>EVKQENRLLNESESSSQGLLGYYFSDLNFQAPMVVTSSTTGDLSIPSSELENIPSENQYFQSAIWSGFIKVKKSDEYTFATSADNHVTMWVDDQEVINKASNSNKIRLEKGRLYQIKIQYQRENPTEKGLDFKLYWTDSQNKKEVISSDNLQLPELKQKSSNSRKKRSTSAGPTVPDRDNDGIPDSLEVEGYTVDVKNKRTFLSPWISNIHEKKGLTKYKSSPEKWSTASDPYSDFEKVTGRIDKNVSPEARHPLVAAYPIVHVDMENIILSKNEDQSTQNTDSQTRTISKNTSTSRTHTSEVHGNAEVHASFFDIGGSVSAGFSNSNSSTVAIDHSLSLAGERTWAETMGLNTADTARLNANIRYVNTGTAPIYNVLPTTSLVLGKNQTLATIKAKENQLSQILAPNNYYPSKNLAPIALNAQDDFSSTPITMNYNQFLELEKTKQLRLDTDQVYGNIATYNFENGRVRVDTGSNWSEVLPQIQETTARIIFNGKDLNLVERRIAAVNPSDPLETTKPDMTLKEALKIAFGFNEPNGNLQYQGKDITEFDFNFDQQTSQNIKNQLAELNATNIYTVLDKIKLNAKMNILIRDKRFHYDRNNIAVGADESVVKEAHREVINSSTEGLLLNIDKDIRKILSGYIVEIEDTEGLKEVINDRYDMLNISSLRQDGKTFIDFKKYNDKLPLYISNPNYKVNVYAVTKENTIINPSENGDTSTNGIKKILIFSKKGYEIG[7x];> MNEHYTESDIKRNHKTEKNKTEKEKFKDSINNLVKTEFTNETLDKIQQTQDLLKKIPKDVLEIYSELGGEIYFTDIDLVEHKELQDLSEEEKNSMNSRGEKVPFASRFVFEKKRETPKLIINIKDYAINSEQSKEVYYEIGKGISLDIISKDKSLDPEFLNLIKSLSDDSDSSDLLFSQKFKEKLELNNKSIDINFIKENLTEFQHAFSLAFSYYFAPDHRTVLELYAPDMFEYMNKLEKGGFEKISESLKKEGVEKDRIDVLKGEKALKASGLVPEHADAFKKIARELNTYILFRPVNKLATNLIKSGVATKGLNVHGKSSDWGPVAGYIPFDQDLSKKHGQQLAVEKGNLENKKSITEHEGEIGKIPLKLDHLRIEELKENGIILKGKKEIDNGKKYYLLESNNQVYEFRISDENNEVQYKTKEGKITVLGEKFNWRNIEVMAKNVEGVLKPLTADYDLFALAPSLTEIKKQIPQKEWDKVVNTPNSLEKQKGVTNLLIKYGIERKPDSTKGTLSNWQKQMLDRLNEAVKYTGYTGGDVVNHGTEQDNEEFPEKDNEIFIINPEGEFILTKNWEMTGRFIEKNITGKDYLYYFNRSYNKIAPGNKAYIEWTDPITKAKINTIPTSAEFIKNLSSIRRSSNVGVYKDSGDKDEFAKKESVKKIAGYLSDYYNSANHIFSQEKKRKISIFRGIQAYNEIENVLKSKQIAPEYKNYFQYLKERITNQVQLLLTHQKSNIEFKLLYKQLNFTENETDNFEVFQKIIDEK

Following assembly, the anthrax protective antigen (PA) forms an oligomeric translocon that unfolds and translocates either its lethal factor (LF) or edema factor (EF) into the host cell. The toxin functions as a binary A2B toxin, with enzymatic A factors, lethal factor (LF, 91 kDa) and edema factor (EF, 89 kDa), and a cell binding B factor, protective antigen (PA, 83 kDa). Within the endosomal compartment, the acidic environment induces a conformational change in the PA, resulting in the formation of a β-barrel channel that can insert itself into the endosomal membrane. The first α helix and β strand of LF and EF unfold and dock into a deep amphipathic cleft, called the α clamp, which resides at the interface of two PA monomers.

The available space on the heptameric PA channel for EF binding can only accommodate up to three EF molecules due to steric hindrance. Indeed, 2D classification of cryo-EM images of PA channel bound with EF showed that the EF binding varies in different classes, suggesting that the space is not fully occupied. Therefore, we used a symmetry expansion method in Relion for 3D classification and were able to resolve the asymmetrically attached EF. Unlike LF, all the domains of EF are well resolved in our channel complex structures. Upon PA binding, these disordered residues of EF (residues 20–30) refold into an α-helix (EFN α1) and bind within the α-clamp site. β1 (Leu33 to Lys35) of EFN forms parallel β-sheet with β13 (Leu203 to Pro205) of PAN. LF α1 is angled downward towards the pore in the α-clamp site, while the amino-terminal end of EF α1 is elevated ~2.9 Å as measured using the carbonyl groups on LF Glu34 and EF Glu24. This elevation in EF α1 appears to be caused by a change in the orientation of PAN Phe464. The phenyl ring in PAN Phe464 is positioned outwards toward the bound EF α1. This change in the orientation of Phe464 appears to restrict EF α1 in its elevated conformation in the α-clamp site. While in the PA7-bound EF structures, the HD domain contributes to a new conformation by bridging the PABD and ACD.>MVSLPVVLIADKLAPSTVAALGDQVEVRWVDGPDRDKLLAAVPEADALLVRSATTVDAEVLAAAPKLKIVARAGVGLDNVDVDAATARGVLVVNAPTSNIHSAAEHALALLLAASRQIPAADASLREHTWKRSSFSGTEIFGKTVGVVGLGRIGQLVAQRIAAFGAYVVAYDPYVSPARAAQLGIELLSLDDLLARADFISVHLPKTPETAGLIDKEALAKTKPGVIIVNAARGGLVDEAALADAITGGHVRAAGLDVFATEPCTDSPLFELAQVVVTPHLGASTAEAQDRAGTDVAESVRLALAGEFVPDAVNVGGGVVNEEVAPWLDLVRKLGVLAGVLSDELPVSLSVQVRG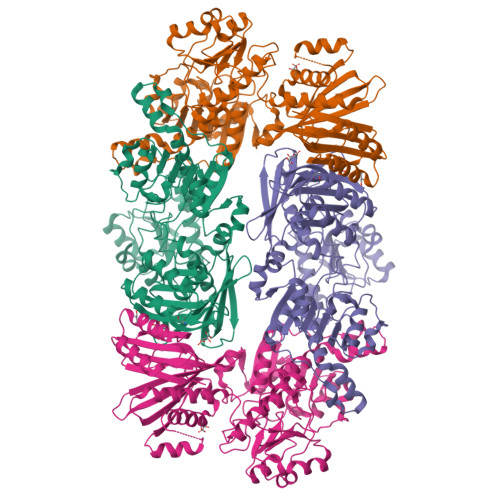ELAAEEVEVLRLSALRGLFSAVIEDAVTFVNAPALAAERGVTAEICKASESPNHRSVVDVRAVGADGSVVTVSGTLYGPQLSQKIVQINGRHFDLRAQGINLIIHYVDRPGALGKIGTLLGTAGVNIQAAQLSEDAEGPGATILLRLDQDVPDDVRTAIAAAVDAYKLEVVDLS[2x]>MKILADKVALVTGSGSGIGLAVALAYGKEGAKVVISDINEQAGNETVKQIESLGGEAVFFKADSSSPADNEALVGYAVKTFGRLDIACNNAGIGGEAALTGDYSLDGWKKVIDINFNGVFYGCKYQIEAMERNGGGVIVNMASIHGTVAAPMSSAYTSAKHAVVGLTKNIGAEYGQKNI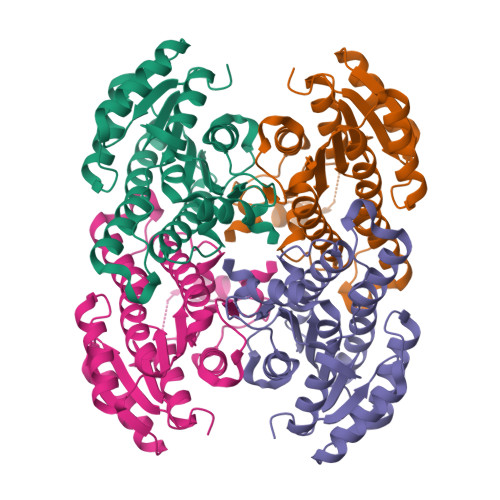RCNAVGPGYIDTPLLAKLDKEHINALISKHPIGRLGKAEEVAELVLFLSSDKSSFMTGGYYLVDGGYTAV[2x]Our structural and functional analysis of the chaperonin ɸEL from the bacteriophage EL of P. aeruginosa revealed that the protein is ATPase active and functions in aggregation prevention of denatured proteins. ɸEL forms tetradecameric double ring complexes, which dissociate into a population of single rings in the presence of ATP and at physiological salt concentration. As anticipated, the ɸEL subunits displayed the typical three-domain architecture of chaperonins, composed of an equatorial domain (residues 2–130 and 425–552), an intermediate domain (residues 131–188 and 388–424), and an apical domain (residues 189–387). The domain structures of ɸEL differ from those of GroEL by numerous insertions and deletions, which alter the putative substrate-binding cleft and the contacts at the ring-ring interface. Our functional data rather suggests that the chaperone mechanism of ɸEL is encapsulation independent, and represents an evolutionary precursor of the more complex encapsulation mechanisms used by the group I and II chaperonins.

To obtain the solution structure of apo-ɸEL, we next performed cryo-EM and single particle analysis. Symmetry-free 3D class averaging indicated a tetradecameric double-ring structure with C2 symmetry. Refinement of the particles resulted in a density map at 3.45 Å resolution, which allowed construction of an atomic model. Apo-ɸEL has an open structure with a ring opening diameter at the apical domains of ~65 Å. In the apo-state, ɸEL is a double ring with six of the seven subunits per ring assuming alternating states (conformations II and III) and one subunit in conformation I. The putative SP binding sites in the apical domains of subunits A, C and E are partially occluded. In all subunits of ɸEL the tip of the αA-β2 loop in the equatorial domain is moved away from the nucleotide binding site as in chains B and D of crystal form II. Other nucleotide binding elements such as the P-loop (residues 79–86) and the β17-β18 hairpin (residues 503–512) are also moved outward (~1.5 Å) in the apo structure. These local conformational changes might facilitate ATP-binding. Similar to group II chaperonins and unlike the staggered subunit contacts in group I, the ring-ring interface of apo-ɸEL is formed by two-fold symmetrical contacts between subunits.

>[14x]MSQTLLVHGKDAQGIIKQVLSEVYDAVTSTMGPNGQLVMIKNGVSTKTTKDGVTVARSIRFADEAHELVNRVITEPATKTDEECGDGTTTTIMLTHALYHLFKDFPGFQHHRNIEDLVERVIQRLESMAIRVEVDDPRLYQVALTSSNQDEKLARLVSELYANNKGSYPDIELKEGVNFEDQIEQTTGRTIRMFYANPWFAKGHQGGVTELTGFTAFVIDRRIDKEDTQKLIDGVNHLVKTHKQHLALPILLIARSFEEAANSTLMQLNAAHPTLVEDGRPWLIPLSTPVGGAIGTSELQDIAVMLNAPMLSDVADLTKLDTHSINGQHGQLELGGNRSILKSTTPKDEDRIEQHARGIEELLEGFSLSDKFSVRARYNERRIRTLRGKLITISVGGETYSEVKERVDRYEDVVKAIRSALENGILPGGGVSLVKAVFGTIKEGLEDKDQSAEFAKRYINSGIANELMRLSTIQHKLLFKDTALYKENGSFHFNDDWLNTPTVMNLATGEIGTPEGLGIYDTAYASITALKGGLQTAKILATTKTLILGEKLSAVKVR> ADKITTVPVQFAKGAHSAQLKGSFTGYDTIHYTLVAKAGQTMTVKIGGSSNANFNVFAPGAQPGQAEAIGRNDGDGQWQGALP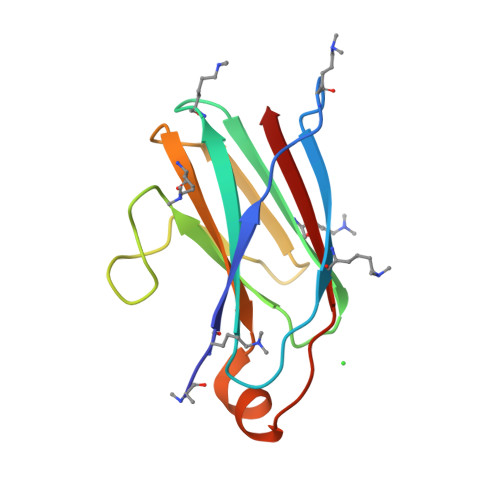ASGKYLIQVYQMRASARRGEQVPHSLAVSIQ>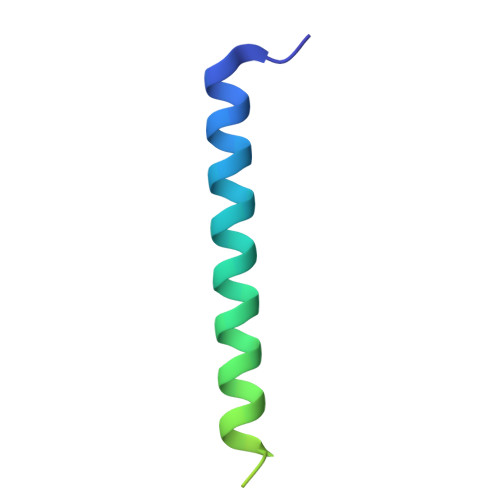 MISDEQLNSLAITFGIVMMTLIVIYHAVDSTMSPKNRTLQVDGGSGGSLEVLFQGPTETSQVAPA One target protein for c‐di‐GMP is PilF, a hexameric ATPase from the thermophilic bacterium Thermus thermophilus important for pilus formation, cell motility, and DNA uptake from the environment. The N‐terminus of PilF contains three homologous so‐called general secretory pathway II (GSPII) domains, GSPII‐A, ‐B, and ‐C. Our recent structures of GSPII‐B (PilF159‐302) showed that the two nucleotide building blocks of c‐di‐GMP are recognized by the protein in a very similar manner through a duplicated amino acid sequence motif. In the GSPII‐B complex with c‐di‐GMP, both c‐di‐GMP phosphodiester groups accept a hydrogen bond from a backbone amide group of a conserved leucine (L168 from the first motif and L197 from the second motif) and from a side chain amino group of a conserved glutamine (Q190 from the first motif and Q218 from the second motif).

To gain insights into the structural basis for the pH‐dependent ligand recognition, we crystallized both the Q190E and the Q218E single‐site mutant of the PilF GSPII‐B domain in complex with c‐di‐GMP using very similar crystallization conditions at pH 7.0. Due to the high‐quality electron density maps for both mutants, their ligand recognition mode could be discerned in detail. In both the Q190E and the Q218E single point mutants, one phosphodiester‐binding pocket can be found in the mutant configuration and the other one in the WT configuration due to the duplication of the c‐di‐GMP phosphodiester binding motifs (Figure S2b‐e). Importantly, the carboxylate groups of the newly introduced glutamate sidechains in either of the two Q/E mutants were found to still point directly towards a non‐bridging oxygen atom of the phosphodiester groups for the carboxamide groups of the native glutamine side chains. The shortest distances between the oxygen atoms of the glutamate carboxylate groups and the phosphodiester groups were found to be 2.6 Å (Q190E) and 2.5 Å (Q218E), respectively, which is well below the sum of the van der Waals radii of the two oxygen atoms. Finally, the lengths of the hydrogen bonds from E190 to the 2′‐OH group of c‐di‐GMP in the Q190E mutant and from E218 to the 2′‐OH group in the Q218E mutant are increased by 0.4 Å if compared to the native sites in both constructs (red numbers). While the c‐di‐GMP binding affinity of the WT protein is similar at pH 4.0 and 8.5 according to ITC titration experiments, both mutants display a drastic increase in ligand affinity at lower pH. The affinity of the Q190E mutant for c‐di‐GMP increased ∼ 20fold with the KD changing from ∼ 800 nM at pH 8.5 to ∼ 40 nM at pH 4.5. Fitting the KD’s measured over a pH range from 4.0 to 8.5 to this formula yielded pKa values of 7.5 and 6.3 for the Q190E/c‐di‐GMP complex and the free Q190E mutant protein, respectively.

>[2x]GSSGEGQKDLKLGELLLQKGWISREALEEALVEEEKTGDLLGRILVRKGLPEEALYRALAEQKGLEFLESTEGIVPDPSAALLLLRSDALRYGAVPIGFQNGEVEVVLSDPRHKEAVAQLLNRPARFYLALPQAWEELFRRAYPQK> MAHHHHHHMISTAETGREPVYSLTGKKIFVAGHTGMVGSAILRRLQHEDCDIIT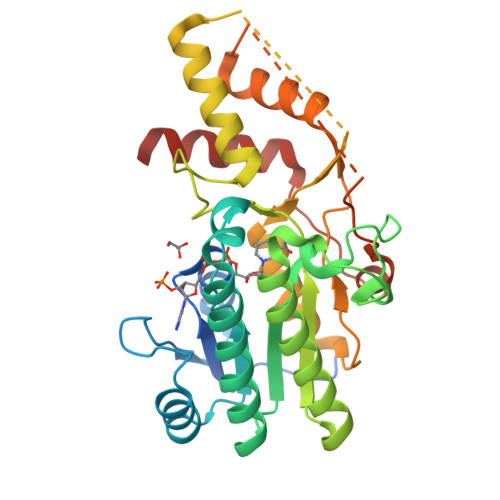AAHSVLDLTRQGPTENFISGHRPDVIIIAAARVGGILANSRFPADFLYDNLAIGMNLIHAAHQIGVERLLWLGSSCIYPRDAAQPLTEDALLTGPLEPTNEAYAIAKIAGLKYAQSCARQFGDRFITAMPTNLYGPNDNFDPTSSHVLPALIRRVHEARMRGAEEVVLWGSGKPLREFLHVDDLADACLHLLRFYNGIEPVNIGSGEEISIKELALTVARIVGYEGRFEHDLSKPDGTPRKLLDTSRIEALGWQPRIHLEDGLRDVYRNWLEETAGSVAA>[2x]MAASLPSTLSFSSAPDEIQHPQIKFSEWKFKLFRVRSFEKAPEEAQKEKDSSEGKPYLEQSPVVPEKPGGQN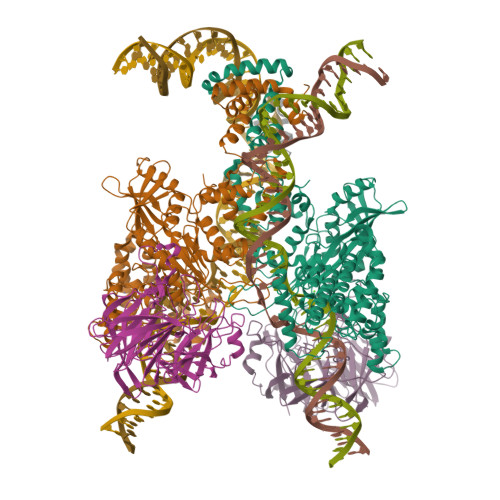SILTQRALKLHPKFSKKFHADGKSSDKAVHQARLRHFCRICGNRFKSDGHSRRYPVHGPVDAKTQSLFRKKEKRVTSWPDLIARIFRIDVKADVDSIHPTEFCHDCWSIMHRKFSSSHSQVYFPRKVTVEWHPHTPSCDICFTAHRGLKRKRHQPNVQLSKKLKTVLNHARRDRRKRTQARVSSKEVLKKISNCSKIHLSTKLLAVDFPAHFVKSISCQICEHILADPVETSCKHLFCRICILRCLKVMGSYCPSCRYPCFPTDLESPVKSFLNILNSLMVKCPAQDCNEEVSLEKYNHHVSSHKESKETLVHINKGGRPRQHLLSLTRRAQKHRLRELKIQVKEFADKEEGGDVKAVCLTLFLLALRARNEHRQADELEAIMQGRGSGLQPAVCLAIRVNTFLSCSQYHKMYRTVKAITGRQIFQPLHALRNAEKVLLPGYHPFEWQPPLKNVSSRTDVGIIDGLSGLASSVDEYPVDTIAKRFRYDSALVSALMDMEEDILEGMRSQDLDDYLNGPFTVVVKESCDGMGDVSEKHGSGPAVPEKAVRFSFTVMRITIEHGSQNVKVFEEPKPNSELCCKPLCLMLADESDHETLTAILSPLIAEREAMKSSELTLEMGGIPRTFKFIFRGTGYDEKLVREVEGLEASGSVYICTLCDTTRLEASQNLVFHSITRSHAENLQRYEVWRSNPYHESVEELRDRVKGVSAKPFIETVPSIDALHCDIGNAAEFYKIFQLEIGEVYKHPNASKEERKRWQATLDKHLRKRMNLKPIMRMNGNFARKLMTQETVDAVCELIPSEERHEALRELMDLYLKMKPVWRSSCPAKECPESLCQYSFNSQRFAELLSTKFKYRYEGKITNYFHKTLAHVPEIIERDGSIGAWASEGNQSGNKLFRRFRKMNARQSKCYEMEDVLKHHWLYTSKYLQKFMNAHNALKSSGFTMNSKETLGDPLGIEDSLESQDSMEF;>MSLQMVTVGHNIALIQPGFSLMNFDGQVFFFGQKGWPKRSCPTGVFHFDIKQNHLKLKPAIFSKDSCYLPPLRYPATCSYKGSIDSDKHQYIIHGGKTPNNELSDKIYIMSVACKNNKKVTFRCTEKDLVGDVPEPRYGHSIDVVYSRGKSMGVLFGGRSYMPSTQRTTEKWNSVADCLPHVFLIDFEFGCATSYILPELQDGLSFHVSIARNDTVYILGGHSLASNIRPANLYRIRVDLPLGTPAVNCTVLPGGISVSSAILTQTNNDEFVIVGGYQLENQKRMVCSLVSLGDNTIEISEMETPDWTSDIKHSKIWFGSNMGNGTIFLGIPGDNKQAMSEAFYFYTLRCSEEDLSEDQKIVSNSQTSTEDPGDSTPFEDSEEFCFSAEATSFDGDDEFDTYNEDDEDDESVTGYWITCCPTCDVDINTWVPFYSTELNKPAMIYCSHGDGHWVHAQCMDLEERTLIHLSEGSNKYYCNEHVQIARALQTPKRNPPLQKPPMKSLHKKGSGKVLTPAKKSFLRRLFD[2x];> MGKGDPKKPRGKMSSYAFFVQTCREEHKKKHPDASVNFSEFSKKCSERWKTMSAKEKGKFEDMAKADKARYEREMKTYIPPKGETKKKFKDPNAPKRPPSAFFLFCSEYRPKIKGEHPGLSIGDVAKKLGEMWNNTAADDKQPYEKKAAKLKEKYEKDIAAYR> GESSLIMNKLKCPHCSYVAKYRRTLKRHLLIHTGVRSFSCDICGKLFTRREHVKQHSLVHKKDKKYK

Very recently, another BTB-ZF protein, ZBTB10 (zinc finger and BTB domain–containing protein 10), has been reported to directly bind a telomeric variant DNA sequence, TTGGGG. Unlike TZAP, ZBTB10 requires two ZF domains to fully recognize the TTGGGG sequence, which represents a different mode of telomeric or telomeric variant DNA binding. Roughly, ZBTB10 follows the well-defined one finger-three base rule of C2H2 fingers, with each of its two C2H2 fingers recognizing 3- or 4-bp of DNA.

Previous studies have revealed that the juxtaposition of Asn or Gln with adenine is a generic mechanism for recognition of the adenine base. Based on the structural mechanism by which ZBTB10 recognizes the TTGGGG sequence, we rationally mutated Arg767 to either asparagine or glutamine and performed ITC assays to check their DNA-binding affinities. We found that the Arg767Asn mutant resulted in severely reduced affinities for both the TTAGGG and TTGGGG sequences. However, the Arg767Gln mutant (referred to as ZBTB10 ZF1–2R767Q) bound to the TTAGGG probe with an obviously higher binding affinity compared with the TTGGGG probe, indicating its preference for telomeric DNA binding. Next, we solved the structure of ZBTB10 ZF1–2R767Q in complex with the TTAGGG sequence. The G-strand sequence of the oligo is “TTAGGGTTATA,” and the C-strand sequence is “ATATAACCCTA”. We determined the structure in the P1 space group to 1.9 Å resolution, with one ZBTB10 ZF1–2R767Q protein binding one DNA duplex in each crystallographic asymmetric unit. We observed that the recognition pattern of G4G5G6T7T8 was preserved very well. Furthermore, Gln767 expectedly donates one hydrogen bond to the adenine N7 atom and accepts one hydrogen bond from the N6 atom of A3, thus conferring the preference of TTAGGG by the Arg767Gln mutant. Furthermore, the binding specificity is also proven by a cocrystal structure. These results raise the possibility that C2H2 finger proteins can employ the well-defined one finger-three base rule to specifically recognize the TTAGGG sequence, and there may be more C2H2 finger proteins functioning in telomeres.Here we focus on the prokaryotic Argonaute AfAgo from Archaeoglobus fulgidus DSM4304. Although phylogenetically classified as a long-B pAgo, AfAgo contains only MID and catalytically inactive PIWI domains, akin to short pAgos. We show that AfAgo forms a heterodimeric complex with a protein encoded upstream in the same operon, which is a structural equivalent of the N-L1-L2 domains of long pAgos. This complex, structurally equivalent to a long PAZ-less pAgo, outperforms standalone AfAgo in guide RNA-mediated target DNA binding.

Next, we obtained cryo-EM structures of the fAfAgo complex with two variants of gRNA/tDNA heteroduplexes: g30/t51 (30 nt gRNA, 51 nt tDNA, final resolution 2.83 Å) and g17/t17 (17 nt gRNA, 17 nt gDNA, resolution 3.56 Å), and a 2.5 Å crystal structure of fAfAgo bound to a 15 nt 5′-phosphorylated ssDNA oligonucleotide. The nucleic acids resolved in the cryo-EM maps include a 25 bp protein-interacting fragment of gRNA/tDNA heteroduplex in the g30/t51 structure, and the full 17 bp gRNA/tDNA heteroduplex in the g17/t17 structure. fAfAgo proteins in these structures overlay with an RMSD value of ∼1.2 Å. Similarly to RsAgo, fAfAgo binds the gRNA/tDNA heteroduplex in the positively charged cleft, which is formed by both AfAgo and AfAgo-N subunits, forming multiple van der Waals and H-bond interactions to the RNA/DNA backbone. The AfAgo subunit, both standalone and AfAgo-N-bound, anchors the 5′–phosphorylated terminus of the guide strand in a conserved MID domain pocket, disrupts the g1:t1 (the first guide strand and the complementary target strand nucleotides) base pair by placing the g1 adenine and the t1 thymine bases into separated protein pockets, and makes similar contacts to the neighboring g2:t2 and g3:t3 base pairs. Taken together, structures presented here demonstrate that fAfAgo heterodimer preserves the g1:t1 base pair recognition mechanism previously demonstrated for the standalone AfAgo, but unlike the isolated AfAgo subunit, fAfAgo binds the guide/target heteroduplex in a specialized cleft in a similar manner as the structurally related long-B pAgos. Full AfAgo, like other long pAgos, forms a deep groove for interaction with the guide-target duplex that is absent in the standalone AfAgo.

> MMEYKIVENGLTYRIGNGASVPISNTGELIKGLRNYGPYEVPSLKYNQIALIHNNQFSSLINQLKSQISSKIDEVWHIHNINISEFIYDSPHFDSIKSQVDNAIDTGVDGIMLVLPEYNTPLYYKLKSYLINSIPSQFMRYDILSNRNLTFYVDNLLVQFVSKLGGKPWILNVDPEKGSDIIIGTGATRIDNVNLFCFAMVFKKDGTMLWNEISPIVTSSEYLTYLKSTIKKVVYGFKKSNPDWDVEKLTLHVSGKRPKMKDGETKILKETVEELKKQEMVSRDVKYAILHLNETHPFWVMGDPNNRFHPYEGTKVKLSSKRYLLTLLQPYLKRNGLEMVTPIKPLSVEIVSDNWTSEEYYHNVHEILDEIYYLSKMNWRGFRSRNLPVTVNYPKLVAGIIANVNRYGGYPINPEGNRSLQTNPWFL;> MGGSHHHHHHGMASENLYFQGGGGEIPLSSGNVNTPDVRSSGILYINIYPIVNYPETIKVSAIPYYEEFLPGKWKKRIGDLIYLYGYGIENEFDEIDNSNALFGKIFRKYLLDILSENIATPWQLKELGSTLRLVKEITENYEFSNIIKLQYELIINVHHWQNTNFGIIVDLKINILDRENNQRISYTKIKDKYGESVKKKIWVSVQAFHRHLTPEGKKYATAMRDKFNLLTGLLKEAFGSSEDEKTFSTPDGEIKIVFKPLEIVEVSNNDGI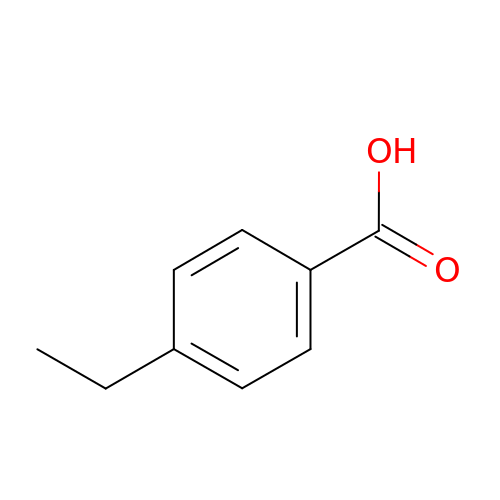4-ethylbenzoic acid | C9 H10 O2 | ZQVKTHRQIXSMGY-UHFFFAOYSA-N> GAMATSVLIVEDEESLADPLAFLLRKEGFEATVVTDGPAALAEFDRA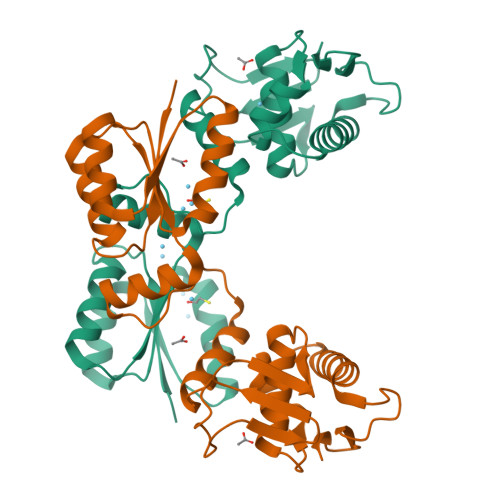GADIVLLDLMLPGMSGTDVCKQLRARSSVPVIMVTARDSEIDKVVGLELGADDYVTKPYSARELIARIRAVLRRGGDDDSEMSDGVLESGPVRMDVERHVVSVNGDTITLPLKEFDLLEYLMRNSGRVLTRGQLIDRVWGADYVGDTKTLDVHVKRLRSKIEADPANPVHLVTVRGLGYKLEG THYMIDINE-5'-TRIPHOSPHATE | C10 H17 N2 O14 P3 | 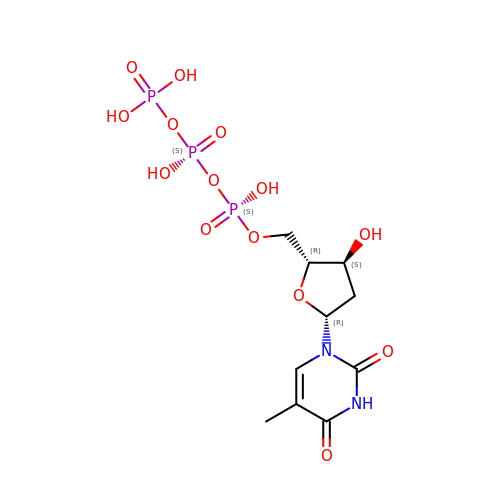NHVNXKFIZYSCEB-XLPZGREQSA-N> MSSDLAAELGFDPALKKKKKTKKVIPDDFDAAVNGKENGSGDDLFAGLKKKKKKSKSVSADAEAEKEPTDDIAEALGELSLKKKKKKTKDSSVDAFEKELAKAGLDNVDAESKEGTPSANSSIQQEVGLPYSELLSRFFNILRTNNPELAGDRSGPKFRIPPPVCLRDGKKTIFSNIQDIAEKLHRSPEHLIQYLFAELGTS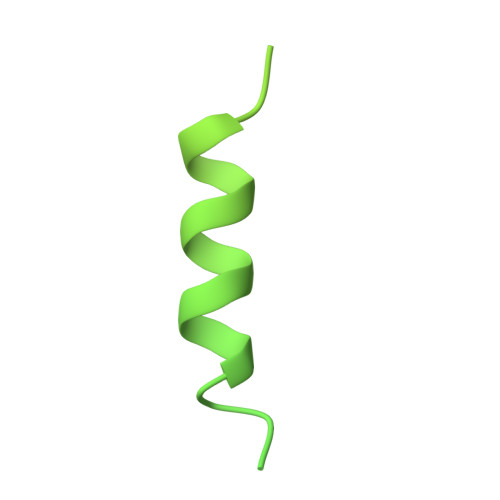GSVDGQKRLVIKGKFQSKQMENVLRRYILEYVTCKTCKSINTELKREQSNRLFFMVCKSCGSTRSVSSIKTGFQATVGKRRRM> CNCKAPE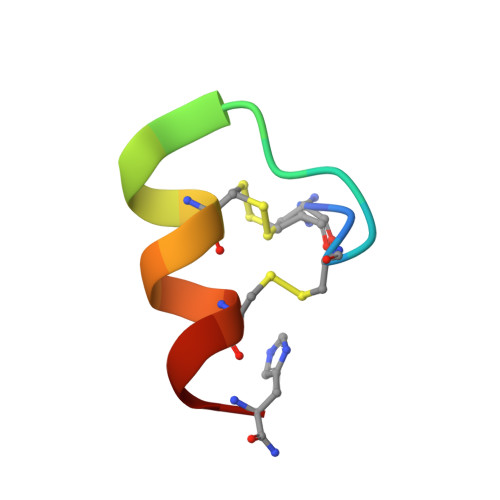TFLCYWRCLQH> MDSLEKIKEEVISCKKCKLW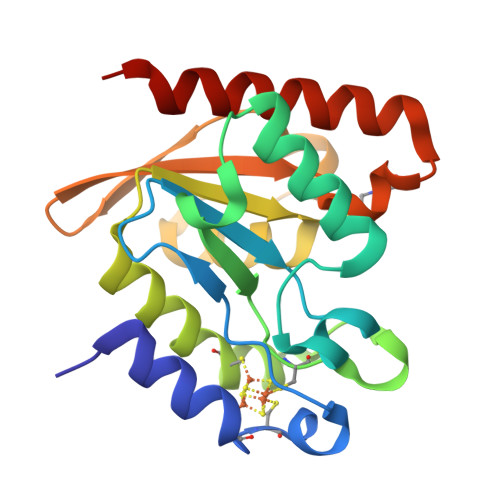QFRTNAVPGEGYPKAEIMFVGEAPGENEDKEGRPFVGAAGKLLTQMIKEILGLERDQVFITNVVKCRPPNNRDPEEDEITACSPYLDRQIDIIMPKIIVTLGRHSTKYIFSKMGENFSSITKVRGKSYVWKYKEKEIIVFPTYHPAAALYNPNLRKILEEDFKKIRELAITPKR>ACVF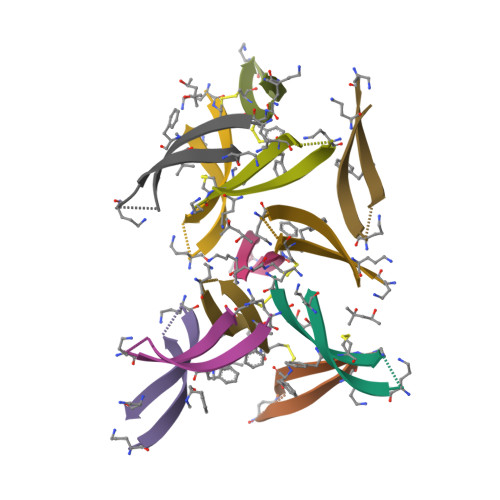FCEDAAXIGLAV[6x]> SQKLDDVDPLVTTNFGKIRGIKKELNNEILGPVIQFLGVPYAAPPTGEHRFQPPEPPSPWSDIRNATQFAPVCPQNIIDGRLPEVMLPVWFTNNLDVVSSYVQDQSEDCL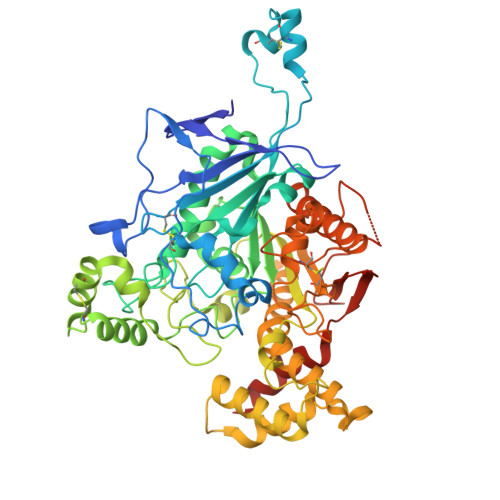YLNIYVPTEDVKRISKECARKPGKKICRKGDIRDSGGPKPVMVYIHGGSYMEGTGNLYDGSVLASYGNVIVITVNYRLGVLGFLSTGDQAAKGNYGLLDLIQALRWTSENIGFFGGDPLRITVFGSGAGGSCVNLLTLSHYSEGLFQRAIAQSGTALSSWAVSFQPAKYARILATKVGCNVSDTVELVECLQKKPYKELVDQDVQPARYHIAFGPVIDGDVIPDDPQILMEQGEFLNYDIMLGVNQGEGLKFVENIVDSDDGVSASDFDFAVSNFVDNLYGYPEGKDVLRETIKFMYTDWADRHNPETRRKTLLALFTDHQWVAPAVATADLHSNFGSPTYFYAFYHHCQTDQVPAWADAAHGDEVPYVLGIPMIGPTELFPCNFSKNDVMLSAVVMTYWTNFAKTGDPNQPVPQDTKFIHTKPNRFEEVAWTRYSQKDQLYLHIGLKPRVKEHYRANKVNLWLELVPHLHNLND>MPVAGSELPRRPLPPAAQERDAEPRPPHGELQYLGQIQHILRCGVRKDDRTGTGTLSVFGMQARYSLRDEFPLLTTKRVFWKGVLEELLWFIKGSTNAKELSSKGVKIWDANGSRDFLD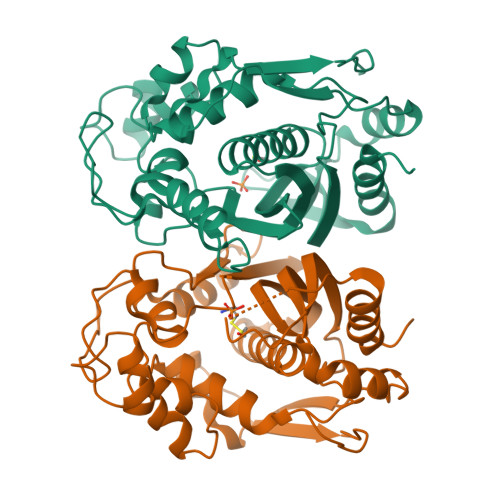SLGFSTREEGDLGPVYGFQWRHFGAEYRDMESDYSGQGVDQLQKVIDTIKTNPDDRRIIMCAWNPRDLPLMALPPCHALCQFYVVNSELSCQLYQRSGDMGLGVPFNIASYALLTYMIAHITGLKPGDFIHTLGDAHIYLNHIEPLKIQLQREPRPFPKLRILRKVEKIDDFKAEDFQIEGYNPHPTIKMEMAV[2x]> C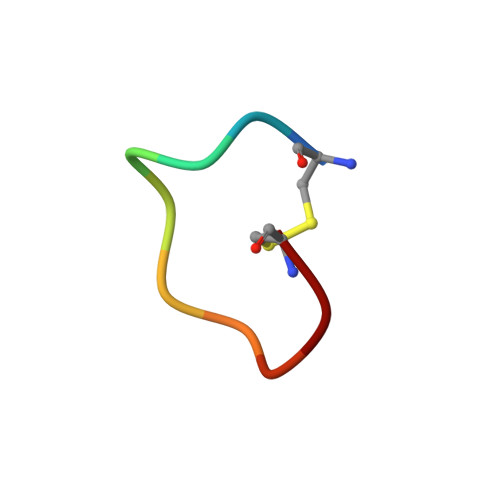PARFAALWC>EQKTRPFTLPNLPLSSLSNSRAPLPISSMGISPDNVQSVQFQNGRCTLDGRLVGTTPVSLSHVAKIRGTSNGTVINLTELDGTPFHPFEGPAPIGFPDLGGCDWHINMTQFGHSSQTQYDVDTTPDTFVPHLGSIQANGIGSGNYVGVLSWISPPSHPSGSQVDLWKIPNYGSSITEATHLAPSVYPPGFGEVLVFFMSKMPGPGAYNLPCLLPQEYISHLASEQAPTVGEA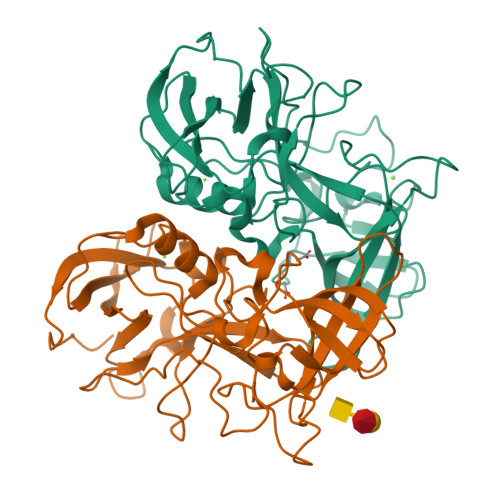ALLHYVDPDTGRNLGEFKAYPDGFLTCVPNGASSGPQQLPINGVFVFVSWVSRFYQLKPVGTA[2x]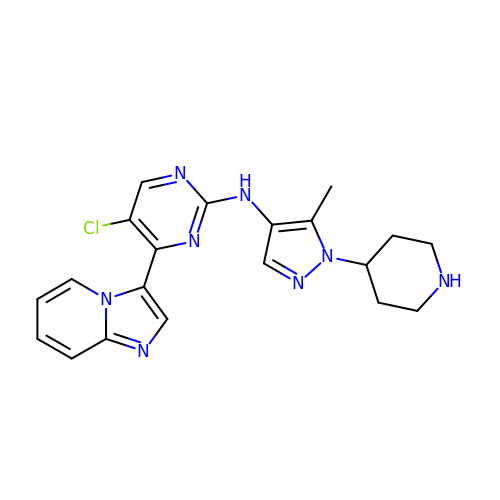5-chloranyl-4-imidazo[1,2-a]pyridin-3-yl-N-(5-methyl-1-piperidin-4-yl-pyrazol-4-yl)pyrimidin-2-amine | C20 H21 Cl N8 | UMHKPLNSKRNIJU-UHFFFAOYSA-N>[2x]MDQRQKLQHWIHSCLRKADKNKDNKMNFKELKDFLKELNIQVDDGYARKIFRECDHSQTDSLEDEEIETFYKMLTQRAEIDRAFEEAAGSAETLSVERLVTFLQHQQRE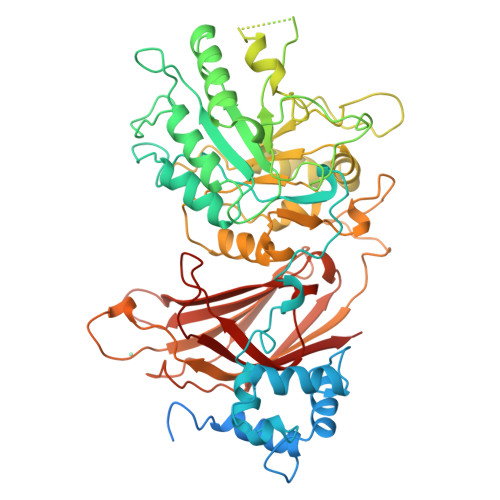EEAGPALALSLIERYEPSETAKAQRQMTKDGFLMYLLSADGNAFSLAHRRVYQDMDQPLSHYLVSSSHNTYLLEDQLTGPSSTEAYIRALCKGCRCLELDCWDGPNQEPIIYHGYTFTSKILFCDVLRAIRDYAFKASPYPVILSLENHCSLEQQRVMARHLRAILGPILLDQPLDGVTTSLPSPEQLKGKILLKGKKLGGLLPAGGENGSEATDVSDEVEAAEMEDEAVRSQVQHKPKEDKLKLVPELSDMIIYCKSVHFGGFSSPGTSGQAFYEMASFSESRALRLLQESGNGFVRHNVSCLSRIYPAGWRTDSSNYSPVEMWNGGCQIVALNFQTPGPEMDVYLGCFQDNGGCGYVLKPAFLRDPNTTFNSRALTQGPWWRPERLRVRIISGQQLPKVNKNKNSIVDPKVIVEIHGVGRDTGSRQTAVITNNGFNPRWDMEFEFEVTVPDLALVRFMVEDYDSSSKNDFIGQSTIPWNSLKQGYRHVHLLSKNGDQHPSATLFVKISIQD>MSELSVATGAVSTASSSIPMPAGVNPADLAAELAAVVTESVDEDYLLYECDGQWVLAAGVQAMVELDSDELRVIRDGVTRRQQWSGRPGAALGEAVDRLLLETDQAFGWVAFEFGVHRYGLQQRLAPHTPLARVFSPRTRIMVSEKEIRLFDAGIRHREAIDRLLATGVREVPQSRSVDVSDDPSGFRRRVAVAVDEIAAGRYHKVILSRCVEVPFAIDFPLTYRLGRRHNTPVRSFLLQLGGIRALGYSPELVTAVRADGVVITEPLAGTRALGRGPAIDRLARDDLESNSKEIVEHAISVRSSLEEITDIAEPGSAAVIDFMTVRERGSVQHLGSTIRARLDPSSDRMAALEALFPAVTASGIPKAAGVEAIFRLDECPRGL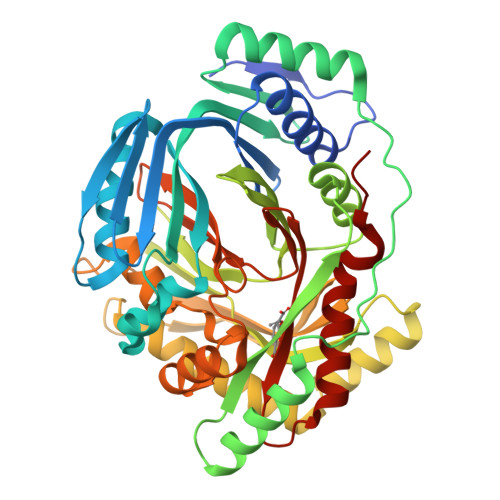YSGAVVMLSADGGLDAALTLRAAYQVGGRTWLRAGAGIIEESEPEREFEETCEKLSTLTPYLVARQ[4x]> MVPISPIETVPVKLKPGMDGPKVKQWPLTEEKIKALVEICTEMEKEGKISKIGPENPYNTPVFACKKKDSTKWRKLVDFRELNKRTQDFWEVQLGIPHPAGLKKKKSVTVLDVGDAYFSVPLDEDFRKYTAFTIPSINNETPGIRYQYNVLPQGWKGSPAIFQSSMTKILEPFKKQNPDIVIYQYIDDLYVGSDLEIGQHRTKIEELRQHLLRWGLTTPDKKHQKEPPFLWMGYELHPDKWTVQPIVLPEKDSWTVNDIQKLVGKLNWASQIYPGIKVRQL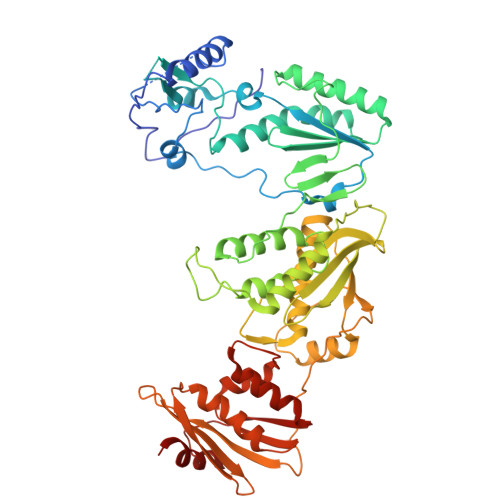SKLLRGTKALTEVIPLTEEAELELAENREILKEPVHGVYYDPSKDLIAEIQKQGQGQWTYQIYQEPFKNLKTGKYARMRGAHTNDVKQLTEAVQKITTESIVIWGKTPKFKLPIQKETWETWWTEYWQATWIPEWEFVNTPPLVKLWYQLEKEPIVGAETFYVDGAANRETKLGKAGYVTNKGRQKVVPLTNTTNQKTELQAIYLALQDSGLEVNIVTNSQYALGIIQAQPDKSESELVNQIIEQLIKKEKVYLAWVPAHKGIGGNEQVDKLVSA>[2x]EEVRQFRRLF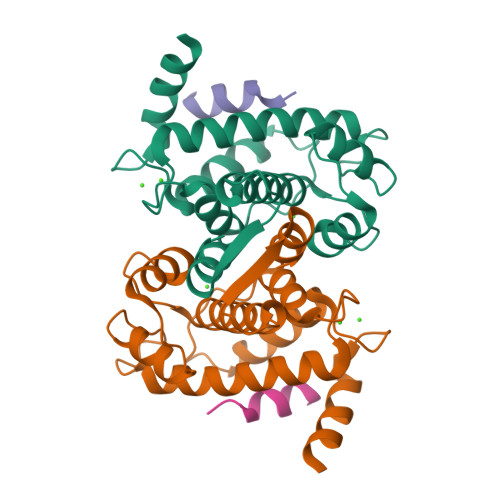AQLAGDDMEVSATELMNILNKVVTRHPDLKTDGFGIDTCRSMVAVMDSDTTGKLGFEEFKYLWNNIKKWQAIYKQFDVDRSGTIGSSELPGAFEAAGFHLNEHLYSMIIRRYSDEGGNMDFDNFISCLVRLDAMFRAFKSLDKDGTGQIQVNIQEWLQLTMYS;>DAIDALSSDFT[2x]6-[(1Z)-3-fluoro-2-(hydroxymethyl)prop-1-en-1-yl]-1,5-dimethylpyrimidine-2,4(1H,3H)-dione 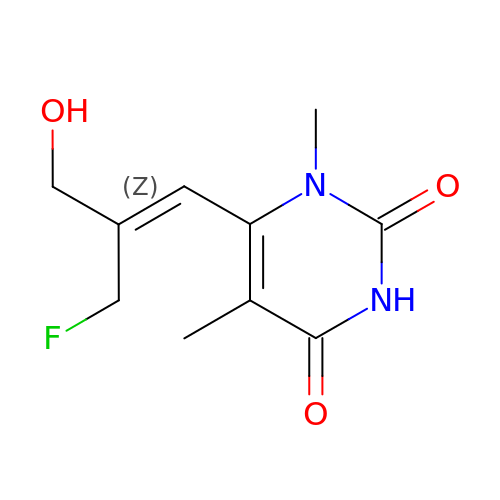| C10 H13 F N2 O3 | NEZZLCCSEJKABY-XVNBXDOJSA-N>MDFQDYIQSLKKDFKLVKINDHTYILHKNKKTLELTPDKMYNIQEINDILNVSYPDISYDRNLEDLGSKNKGILNGFGNVGEDDLHPQIGRRKGKKKGAIFSPEEFKEEEDSDGIDKTDIFPLKKKRDPDSDHFKKTGGDDDNPFLY[2x];>[2x]MFLDTHKQLTLFTSEGKLDQCDNALKAATQGSLSVGCVSENGVVLASLKESNNLVILSEYKKIYQISPNLGITYSGCQPDFRIQYNLSLKISEEYTDIYSTNIPIRLFVEQFSRQIQEYTIKKGYRPFGTLLLIVGDNKMYRVDPSGSYTSLQVGTIGREYTESGRLLERRKGMLDDNISTCVECIREYCGRSVKSEDIDIGVYRGQEFRVYSKEEVQEVFDSINKI;>MSSNTFTEEGRLLQTEYAIKNVSKGGTIIGLVCKDGVILLGINKTELLDEREKIYKINPKVYVSVSGLFGDAMLLKKYGQVKAQDFLYEFDYDCDIDRICNFISEKKQLFTQYNSTRPFGFSFIYAGMKNNKFKLCSTDPSGTINEWKGVCFGENEDAINNGLRNDFPDEEMDMERGLFEIFKILSKVTECSAKDHKKYEILYFKNEESRFLEFEEIENILLRIEEEKNKK[2x];>[2x]MEYENALGIFSPDGRLIQVEYAQQASEQGSLVVFSSDTNEICLSIETKTHNKMLIDQNKLLPVDKDLNIWYTFSGIKPDSYKVLNEARLICRNYKIKTGTNISFDELAYELSLYKQKFTLDSSMRPFGIRSILLQVKDMAKIYVLEPDGNYSEYKCGAVGQKSVSVCEYLEKCEEEDIIFRSVSGLGTVVQSDKNKVMSYVISKDEIRRVEDETVSQIISTVSVK;>[2x]MSIVSRQNANTYSAEGRLYQVEYAMQAMNLGTSSIGIKTKDYVLLASEKKIISKLQNPSSVKKHYRVYDHIALGFSGISADVKTIVDKSRNFAINHEYLYDENCKVERLLEHLADLSLNFDKKEADEKIFSRPFGASLLIIGYDTEPRLFSLDPSGSYLEYHAKAIGSGSEVIENMLEQEFDPNVDINSGLKNILNMLSKVMKDKINNFNVEITAITKNECKILTPEEIEQFLE;>[2x]MNSQTDYTNYIIFNPEGKIKQLEFINNTVQLGSTVVALKNKSFGVFVTYNEKRSKFALQQKKIFPINSKSLFSFSGITNDGTKIVKYLKNSTVFENIRKGRDIHPIHVFDDLCYSACIRTLTNGNRLYGVQGLLLTDYQGISLVLFDPKGSAKEVRGMSIGSRSQSCRTILEDECDKFEEYNKEELVRLGIKALRNAYPETGVLNKDNVDIWILETNQESKQIKSEEYLQ;>MAILDVDTVYTNTGDILQIGYAQKAADNGNTAICMKNKKGLIMIAEKPIESKLYVSEKNFRIKKVNNSIFQISSGIETDLVYINENLKNNLISEKHSNDMDVSHESVRNQIVNIIHQFTRYSGVRPIGINLLTCSKYKNEYKILQTDCTGKSLFFKSSVIGKGSRIVKTELEKLNLENMEIRDLVENGIRILYKSYDPLKDKPFDIEIGIMCEETNGEFVRLEKNQYSEIIEKYKDFSVDGEE[2x];>MSIKDEIYNIFNADGKILQIEYGLEAVNKSLPLVVLKNKNMIVCAAKKNQGHLLEDEVQTSFQPIYPNLYSAFTGNWADVFYVNSKAKDLAHYASYKLGFSVTPDILCRKLADELQPLIQSTGERAPAFAGALFGFDNGKPVVYMTNISAVCYPVYGSMVGSKNQNMYKYVEKYYNEDIEDEKLFEVAVGGLLESLGENSVYQEMEVAYLRNGEVLKYLDDKEIESLLLSIADK[2x];>[2x]MFTKTGTTIVGVKYKGGVVICADTRSTSGPIVADKNCSKIHYISDNIQACGAGTSADITRVTRKASKVLSIFSKTYNRLPRVSHCVRTCQLHLHPYQGHISAALVVGGVDDTGAHLYDVYPHGSSNSVSYTALGSGSLAAISILEAGYKDMNREEAMELACAAIEAGIMNDLYSGSNIDVCVISQEGREMFRNYKKVGVRNEVPKFQYPRSSVKILKEDIYKYIEEK;>[2x]MSDISQHYGGSLLAMIGKSSVAFLSDKRLGSGPISVSKNFTKIYSLTPRLFFGFTGLVSDGEMLFKKIRKNYNLFVQDNNKDMEPSELSNMISYILYQKRLQPYYVAVIVCGMTLDKKPYASSMDCIGAMKETSEFVTSGTASKNLMGLSEALFYPEMEDEDLFTTSVQTFLNSSDRDTFGGMGFECLLINPEGYKRREFVGRCD;>MESSVALKGNDFVIIGTDSSVKNSYLVLKREEDKFYNINNKVVFTYLGDQGDAFRTSSFINEKLVYEEIQNNVEITPKVTANVIQKTLYDNLRSHPKNCYFLVGGLSQDGPELYSVDLYGSLHENDFMAVGISTYFCYGVLDKEYHKNITKEDGIKIIQKCFDVLKQRCSVDISNIEIKIVSKEGVETINKVL[2x];>MEKLFTGDIMEIQNTKVDSAFMKNKIVPYKGTTTLAFIFQGGMVIAVDSRASAGSYIASQNVHKVIRVNKHLIGTMAGGASDCYFWEKKMGLYAKLYELKNNKRISVSAASMYLSNCVYSYKGQGLSLGSMVCGYDGDKPVIYYVDDAGQRLSGDLFSVGSGSTIAYGVLNESYRFDLTKEEALNLGKKAIWHATHRDAYSGGNVNLYFMDKNGWEHLGTFDVDKFEQ[2x];>MFTLQANTKDQIIKDLNIGDLTIRDLNIKDLNIGDSSTVNLFKVDIPLLSNEIPLDFTFDNLPSNKKEIFESFDSFTDFVEGKTKSQESKFNPYEDNSGSTVSIRLNNSIIIAADTRHCSEMGIYSRNTSKIFRIGDFLLTITGFYADGYELYNRLKYQVQIYESFNKISIHSLANLASKIMYSKRLFPYYSYVTLSGFEGDNPYVYSFDCLGHFEEVDSVCNGSGSPLIQPLLDSTIEKKNWAGENYEVTEEYVKDIVRRGFNAASERDVKTGDNVEIWIIKKDGMTKEYERLRQD[2x];>[2x]MKNFVIGSGVISLRYKNGVITCTDTQASYGNLCKFNDVRRIFRLSSNTLISLSGEISDIQFLMNELNKLNESDPVKMSPRGYLNLVQGILYNKRSRVEPLNVSVSIVGVDDDDFLVSCVNHLGNFYEDNIVCTGLSNMIALPFLRTCNVLDLERDEAISLVEKAMTVMCYRSCRSSNRIQIGVVEKGLVDISDPYVLNTDWQVGHNEEEIVL;>[2x]MVAYDNKNNEGFSPNLPEMTGTTIMAVKYADGILIGADCRTSMGTYVSSRFTDKLTKISDNIYCCRSGSAADTQAITQYITELVQRSSFIDKEIPSVKKAAMAAKDIIYRYPNMLAGLIIAGYDTKPRIFNISLGGTMTEAEWQIGGSGSAYIYGLCDTTFKPNMNLEEALEFVKLAVTCAIKRDNASGGCIRMASITREGVQRFFYSGDKILNST

Proteasomes, proteolytic complexes expressed in all known eukaryotes, play a key role in this process by degrading undesirable and misfolded proteins. While the RP is responsible for substrate recognition, deubiquitination, unfolding, and translocation, the CP houses the proteolytic active sites that hydrolyze targeted proteins. Similar to typical eukaryotes, microsporidian proteasomes are composed of 28 proteins in a C2-symmetric α1–7β1–7/β1–7α1–7 arrangement. The 20S structure described in this work is the most minimized eukaryotic proteasome studied to date and reveals that microsporidia have deleted many of the insertions that differentiate individual α and β subunits.

To study proteasomes derived from the dormant state, we ruptured spores via bead-beating, in the absence of ATP, and performed size exclusion chromatography on the spore lysate. Using 52,679 particles for 3D refinement, we obtained a 2.8 Å map of the 20S CP. Here, we use cryo-electron microscopy (cryo-EM) to study the 20S proteasomes isolated from dormant microsporidian spores and identify a pair of PI31-like (PI31L) proteins symmetrically bound at high occupancy within the 20S central cavity. The identified PI31L of V. necatrix, a small protein of 147 amino acids, fits in the available density. Two PI31L molecules bind with their C-terminal half (residues 76 to 147) symmetrically in the central cavity and occlude all 3 active sites in each ring. The resolved C-terminal portion of the protein starts on β5 and β6 with the two shorter fragments (76-89, 96-107), connected through a disordered linker of 6 amino acids. A short flexible linker connects these shorter fragments to the continuous density corresponding to amino acids 113-147, located on the opposite β-ring. There, PI31L blocks the active sites of β2 and β1 and buries its C-terminal end in binding sites on β7. In the β5 pocket, PI31L bulges out and loops back in on itself, resulting in Phe101, Ile100, Ala99, Asp84, and Leu85 representing P3, P2, P1, P1', and P2', respectively. However, PI31L appears to evade digestion via structural constraints caused by Pro129 in the P4 site, which serve to push the P1 site Asp132 out of the active site and into a region where the angle is suboptimal for nucleophilic attack by the active site threonine.> ADLGHQTLGSNDGWGAYSTGTTGGSKASSSNVYTVSNRNQLVSALGKETNTTPKIIYIKGTIDMNVDDNLKPLGLNDYKDPEYDLDKYLKAYDPSTWGKKEPSGTQEEARARSQKNQKARVMVDIPANTTIVGSGTNAKVVGGNFQIKSDNVIIRNIEFQD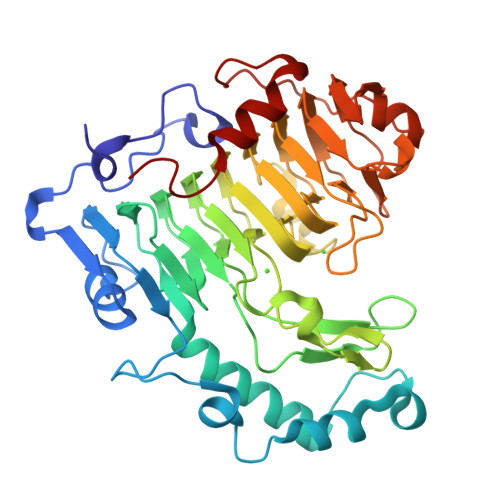AYDYFPQWDPTDGSSGNWNSQYDNITINGGTHIWIDHCTFNDGSRPDSTSPKYYGRKYQHHDGQTDASNGANYITMSYNYYHDHDKSSIFGSSDSKTSDDGKLKITLHHNRYKNIVQRAPRVRFGQVHVYNNYYEGSTSSSSYPFSYAWGIGKSSKIYAQNNVIDVPGLSAAKTISVFSGGTALYDSGTLLNGTQINASAANGLSSSVGWTPSLHGSIDASANVKSNVINQAGAGKLN> XAA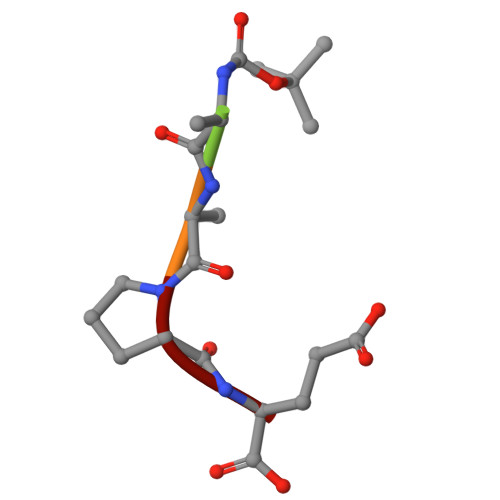PE>MTSFTIPGLSDKKASDVADLLQKQLSTYNDLHLTLKHVHWNVVGPNFIGVHEMIDPQVELVRGYADEVAERIATLGKSPKGTPGAIIKDRTWDDYSVERDTVQAHLAALDLV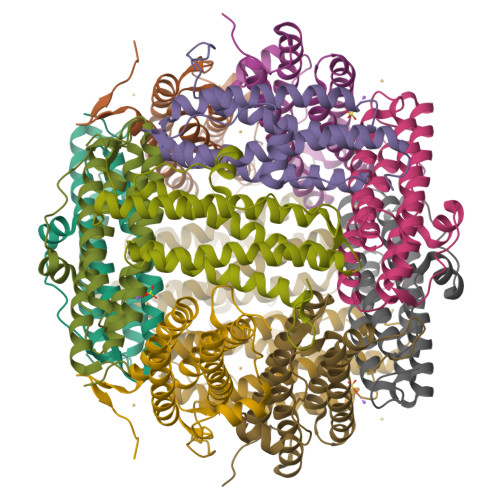YNGVIEDTRKSIEKLEDLDLVSQDLLIAHAGELEKFQWFVRAHLESAGGQLTHEGQSTEKGAADKARRKSA[6x]>GPLGSMSRLPLIGVTACTKQIGLHPYHIAGDKYLRAVVNGAGGLPLIIPALGESIDQAALLDSVDGLLFTG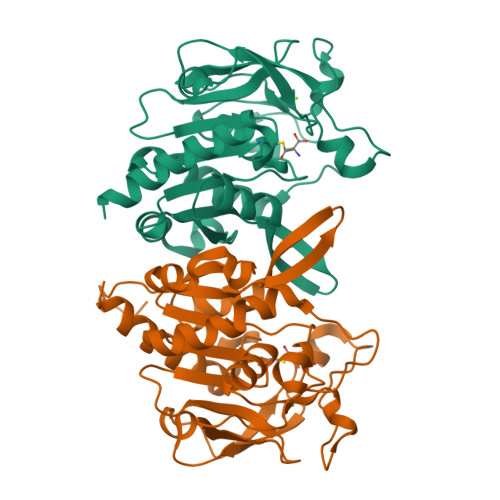SPSNVEPRHYSGPASEPGTLHDSDRDATTLPLVRAAIDAGIPVLGICRGFQEMNVAFGGSLHQKVHEVGTFMDHREPADQPLEVQYAPRHAMHVQPGGVLAGIGLPSEFQVNSIHGQGVDRLAPGLRVEALAPDGLVEAISVEGAKAFALGVQWNPEWQVLTNPNYLAIFQAFGKACSKRAGQR[2x]> GSDLTVSLIPVSGLKAGKNAPSAKIAKLVVNSTTLKEFGVRGISNNVVDSTGTAWRVAGKN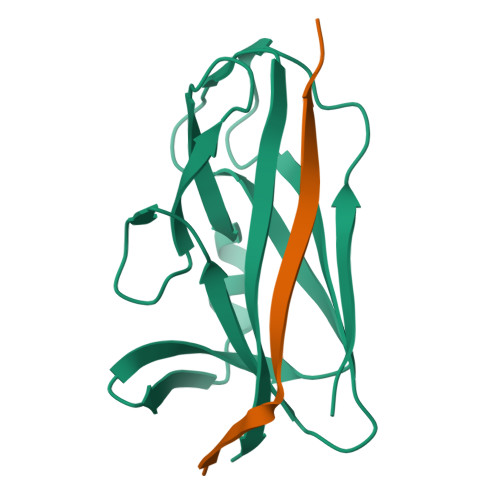TGKEIGVGLSSDSLRRSDSTEKWNGVNWMTFNSNDTLDIVLTGPAQNVTADTYPITLDVVGYQP;> GSFLPNSEQQKSVDIVASSP>MDFSRNLYDIGEQLDSEDLASLKFLSLDYIPQRKQEPIKDALMLFQRLQEKRMLEESNLSFLKELLFRINRLDLLITYLNTRKEEMERELQTPGRAQISAYRVMLYQISEEVSRSELRSFKGGLQEEISKCKLDDDMNLLDIFIEMEKRVILGEGKLDILKRVCAQINKSLLKIINDYEEFSKERSSSLEGSPDEFSNGEELCGVMTISDSPREQDSESQTLDKVYQMKSKPRGYCLIINNHNFAKAREKVPKLHSIRDRNGTHLDAGALTTTFEELHFEIKPHDDCTVEQIYEILKIYQLMDHSNMDCFICCILSHGDKGIIYGTDGQEAPIYELTSQFTGLKCPSLAGKPKVFFIQAAQGDNYQKGIPVETASEEQPYLEMALSSPQTRYIPDEADFLLGMATVNNCVSYRNPAEGTWYIQSLCQSLRERCPRGDDILTILTEVNYEVSNKDDKKNMGKQMPQPTFTLRKKLVFPSD[3x];>[5x]MSAEVIHQVEEALDTDEKEMLLFLCRDVAIDVVPPNVRDLLDILRERGKLSVGDLAELLYRVRRFDLLKRILKMDRKAVETHLLRNPHLVSDYRVLMAEIGED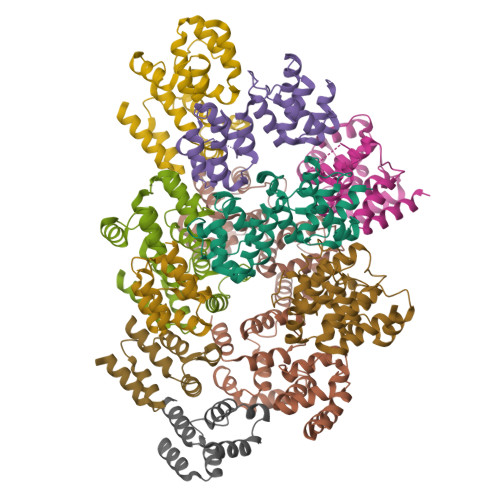LDKSDVSSLIFLMKDYMGRGKISKEKSFLDLVVELEKLNLVAPDQLDLLEKCLKNIHRIDLKTKIQKYKQSVQGAGTS;>[3x]MDPFLVLLHSVSSSLSSSELTELKGLCLGRVGKRKLERVQSGLDLFSMLLEQNDLEPGHTELLRELLASLRRHDLLRRVDDFEAGAAAGAAPGEEDLCAAFNVICDNVGKDWRRLARQLKVSDTKIDSIEDRYPRNLTERVRESLRIWKNTEKENATVAHLVGALRSCQMNLVADLVQEVQQARDLQNRSGAMSPMSWNSDASTSEASLEHHHHHH> XSLSATDKARVKALWDKIEGKSAELGAEALGRMLVSFPQTKIY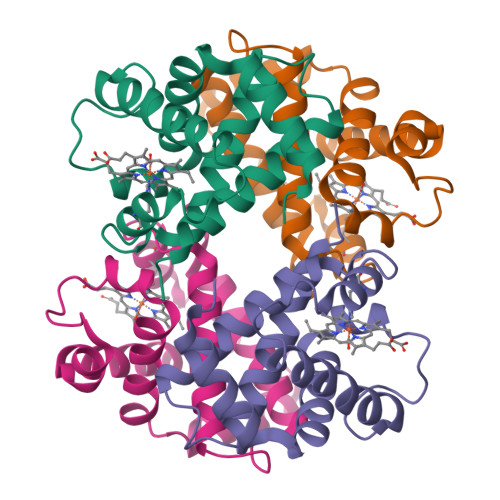FSEWGQDLGPQTPQVRNHGAVIMAAVGKAVKSIDNLVGGLSQLSELHAFKLRVDPANFKILAHNIILVISMYFPGDFTPEVHLSVDKFLACLALALSEKYR;> VDWTDAERAAIKALWGKIDVGEIGPQALSRLLIVYPWTQRHFKGFGNISTNAAILGNAKVAEHGKTVMGGLDRAVQNMDNIKNVYKQLSIKHSEKIHVDPDNFRLLGEIITMCVGAKFGPSAFTPEIHEAWQKFLAVVVSALGRQYH>GAMGSKFSVEEYLVHALQGSVSSGQAHSLTSLAKTWAARGSRSREPSPKTEDNEGVLLTEKLKPVDYEYREEVHWATHQLRLGRGSFGEVHRMEDKQTGFQCAVKKVRLEVFRAEELMACAGLTSPRIVPLYGAVREGPWVNIFMELLEGGSLGQLVKEQGCLPEDRALYYLGQALEGLEYLHSRRILHGDVKADNVLLSSDGSHAALCDFGHAVCLQPDGLGKSLLTGDYIPGTETHMAPEVVLGRSCDAKVDVWSSCCMMLHMLNGCHPWTQFFRGPLCLKIASEPPPVREIPPSCAPLTAQAIQEGLRKEPIHRVSAAELGGKVNRALQQVGGLKSPWRG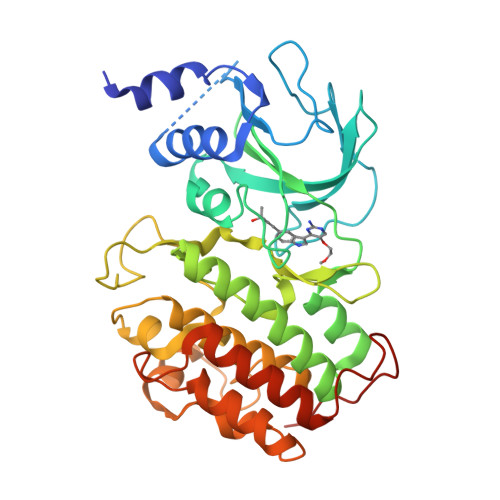EYKEPRHPPPNQA[4x]>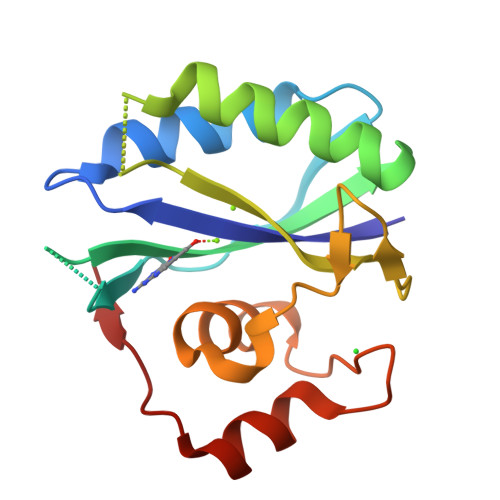TVAYIAIGSNLASPLEQVNAALKALGDIPESHILTVSSFYRTPPLGPQDQPDYLNAAVALETSLAPEELLNHTQRIELQQGRGGPRTLDLDIMLFGNEVINTERLTVPHYDMKNRGFMLWPLFEIAPELVFPDGEMLRQILHTRAFDKLNKW[2x]> MTSHRQSSDTFGGILPSTLSSRYLSIVNQLPEEFSSVVSEMMVHLENIFSLAENFFQAIERFSRTPDLLERNKMSIGVGAEGDSWPCHVSHEAPMGSAQTTENSAKEEDKQVPESAALQHPKFKSTPGPQLPTRRRFLSESDELQDPQPVWDAEPQFCQGFLIQGLWELFMDSRQKNQQEHGGEDSSQESKDSGLCDFKPEPQPRHRNSLSDSADPFLIKSPSALLDYYQEDVSRPQPETQESSGRADKFLKPLSWGSEVLESSCNQPSTALWQLERFTVPQALQKVRVLKHQELLLVVAVSSFTRHVFTCSQSGIKVWNLVNQVAEDRDPESHLKCSVQDNKVYLRTCLLSSNSRTLFAGGYNLPGVIVWDLAAPSLYEKCQLPCEGLSCQALANTKENMALAGFTDGTVRIWDLRTQEIVRNLKGPTNSARNLVVKDDNIWTGGLDACLRCWDLRMAKVSLEHLFQSQIMSLAHSPTEDWLLLGLANGQHCLFNSRKRDQVLTVDTKDNTILGLKFSPNGKWWASVGMGNF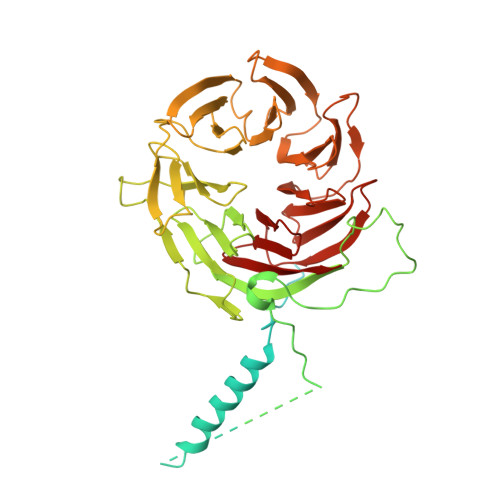ITVHSMPTGAKLFQVPEVGPVRCFDMTENGRLIITGSRDCASVYHIKY> GSRSTVSMSDVFNSPQARSTISAAFGIKPTAGQDVEELLIPKVWVPPEDPLASPSRLAKFLRENGYKVLQPRSLPENEEYETDQILPDLAWMRQIEGAVLKPTLSLPIGDQEYFPKYYPTHRPSKEKPNAYPPDIALLKQMIYLFLQVPEANEGLKDEVTLLTQNIRDKAYGSGTYMGQANRLVAMKEVATGRNPNKDPLKLGYTFESIAQLLDITLPVGPPGEDDKPWVPLTRVPSRMLVLTGDVDGDFEVEDYLPKINLKSSSGLPYVGRTKGETIGEMIAISNQFLRELSTLLKQGAGTKGSNKKKLLSMLSDYWYLSCGLLFPKAERYDKSTWLTKTRNIWSAPSPTHLMISMITWPVMSNSPNNVLNIEGCPSLYKFNPFRGGLNRIVEWILAPEEPKALVYADNIYIVHSNTWYSIDLEKGEANCTRQHMQAAMYYILTRGWSDNGDPMFNQTWATFAMNIAPALVVDSSCLIMNLQIKTYGQGSGNAATFINNHLLSTLVLDQWNLMRQPRPDSEEFKSIEDKLGINFKIERSIDDIRGKLRQLVLLAQPGYLSGGVEPEQSSPTVELDLLGWSATYSKDLGIYVPVLDKERLFCSAAYPKGVENKSLKSKVGIEQAYKVVRYEALRLVGGWNYPLLNKACKNNAGAARRHLEAKGFPLDEFLAEWSELSEFGEAFEGFNIKLTVTSESLAELNKPVPPKPPNVNRPVN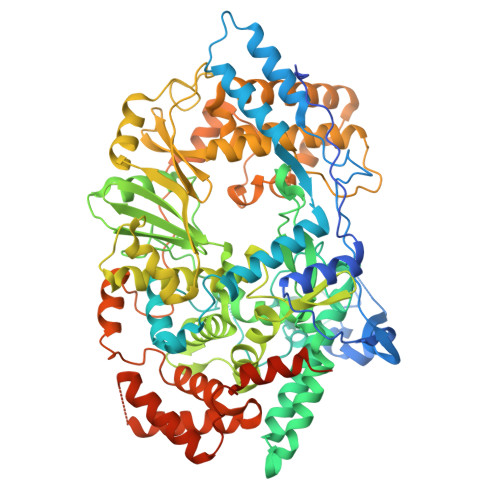TGGLKAVSNALKTGRYRNEAGLSGLVLLATARSRLQDAVKAKAEAEKLHKSKPDDPDADWFERSETLSDLLEKADIASKVAHSALVETSDALEAVQSTSVYTPKYPEVKNPQTASNPVVGLHLPAKRATGVQAALL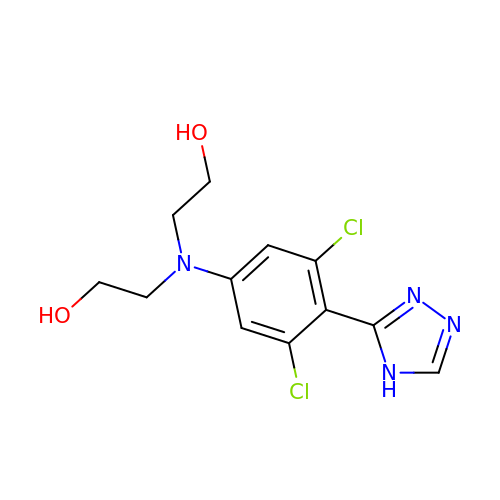2-[[3,5-bis(chloranyl)-4-(4~{H}-1,2,4-triazol-3-yl)phenyl]-(2-hydroxyethyl)amino]ethanol | C12 H14 Cl2 N4 O2 | KTFYALGLEDTFHG-UHFFFAOYSA-N EccC, the motor subunit of T7SS, is essential to assemble a stable membrane complex for the secretion process. It contains a two-pass transmembrane domain, an unknown function domain (DUF), and three Fts-SpoIIIE-like ATPase domains (ATPase1, ATPase2, and ATPase3). In this study, we have provided high-resolution crystal structures of ATPase3 domains of EccC proteins from Mtb, all in complex with ATP. In our structures, ATP and a magnesium ion bind to the nucleotide-binding site in a similar manner.

To determine how MtEsxB is recognized by MtEccCb1-ATPase3, a structure of the complex was determined at 1.98 Å resolution. Only the C-terminal 14 residues of MtEsxB was stable through strongly binding to MtEccCb1-ATPase3 according to the high-resolution density. The first 11 residues form an α-helix while the last three residues form a short loop. Most importantly, it is the side chains of Met98 and Phe100 in MtEsxB that insert into the recognition pocket of ATPase3, which is located in the gap between ɑ2 and β4. The phenyl ring of Phe100 is sandwiched by Asn445 and Phe469, with Leu442, Leu446, Arg449 and Val471 all located within van der Waals distance. Met98 is surrounded by Leu423, Ala425 and Leu442. Additionally, Leu94 is close to ɑ2 and interacts with Glu437 and Ala441. Superposition of the MtEsxB bound and free MtEccCb1-ATPase3 structures showed that the bulge loop moves by ~3.5 Å to allow Gly424 and Ala425 to form interactions with MtEsxB. Thus, the shift of bulge loop could further strengthen substrate binding. A previous report showed that Asp87 in the conserved Yxxx[D/E] motif of MtEsxB is required for secretion, however this residue makes no interactions with MtEccCb1-ATPase3 in our structure.

> GPGSTEQAPPVRVLPERIHLHELDPNPPGPESDYRTRWEIPIGLRETDLTPAHCHMHTNPHLLIFGAAKSGKTTIAHAIARAICARNSPQQVRFMLADYRSGLLDAVPDTHLLGAGAINRNSASLDEAVQALAVNLKKRLPPTDLTTAQLRSRSWWSGFDVVLLVDDWHMIVGAAGGMPPMAPLAPLLPAAADIGLHIIVTCQMSQAYKATMDKFVGAAFGSGAPTMFLSGEKQEFPSSEFKVKRRPPGQAFLVSPDGKEVIQAPYIEPPEEVFAAPPSAG;> GPGSMAEMKTDAATLAQEAGNFERISGDLKTQIDQVESTAGSLQGQWRGAAGTAAQAAVVRFQEAANKQKQELDEISTNIRQAGVQYSRADEEQQQALSSQMGF> QMPTEDE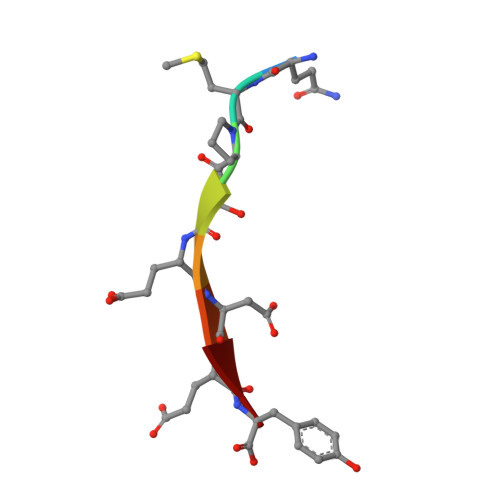Y>[2x]MSEKKDQYPSPGYSEFGATLVDLFSRAAMEMPDRTALHIDDEKISYGLLHSWAEGLADLLHDAGVRKGDRVALRMPPGANAIAAMLGILRAGAAYVPLDIRNPPARNAFIVTDSQVVALVGDPGDIPEYTGPLVTEENVAALRDREAIKDPGPERPGPQDVAYIIYTSGTTGRPKGVPVRHGNVTALFEACSRLFSFSADDRWLLFHSMAFDFSVWEIWGALSTGAELVVLPYWTARTPVETARVVRDRGITVLNQTPTAFGALTT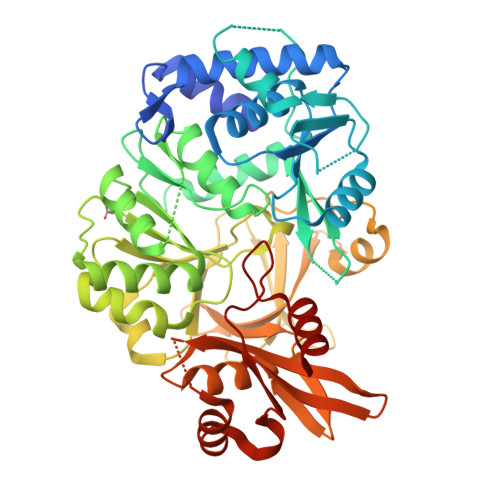AVLGEGIDLPELRYVVFGGEKLTPAVVRPWAKRFGLDRPHLINMYGITETTVHATFHRLTEDDLAAEDSVIGRPLPGFTHRIVTEDGRDAATGEPGELWLAGPQVSEGYLNRPELTAERFTTGPARDGGAPPPRYYHSGDLVSRRAGGDLVYQGRADLQVKLRGHRIELSDVEAAVRTHPAVVDAVVWVHEFAPGDSRLVCAYTAQASEEGTGPDARALRAHVKTVLPSYMQPSQYLALPELPRTINGKADRASVARAFDERR(2S,3R)-2-azanyl-N-[(1R)-2-[3-[6,7-bis(chloranyl)-4-oxidanylidene-quinazolin-3-yl]propanoylamino]-1-[3-[4-(trifluoromethyl)phenyl]phenyl]ethyl]-3-oxidanyl-butanamide | C30 H28 Cl2 F3 N5 O4 | 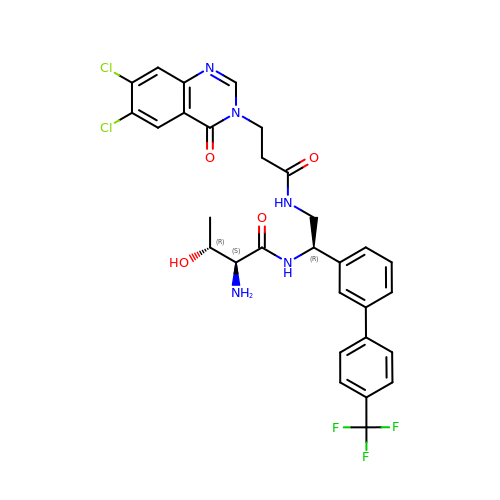MITSAJKYFZWXSM-YDZMPMGISA-N>MKVTFEQLKAAFNRVLISRGVDSETADACAEMFARTTESGVYSHGVNRFPRFIQQLENGDIIPDAQPKRITSLGAIEQWDAQRSIGNLTAKKMMDRAIELAADHGIGLVALRNANHWMRGGSYGWQAAEKGYIGI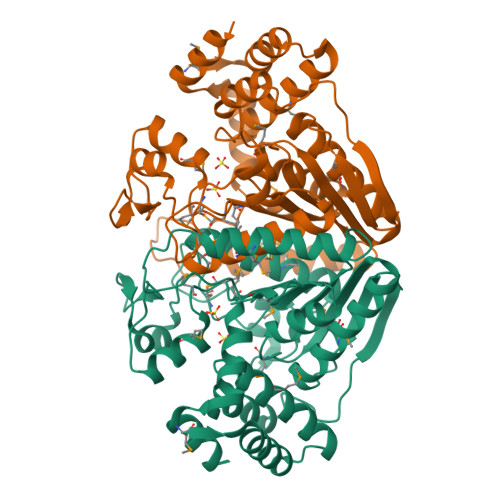CWTNSIAVMPPWGAKECRIGTNPLIVAIPSTPITMVDMSMSMFSYGMLEVNRLAGRQLPVDGGFDDEGNLTKEPGVIEKNRRILPMGYWKGSGMSIVLDMIATLLSDGASVAEVTQDNSDEYGISQIFIAIEVDKLIDGPTRDAKLQRIMDYVTSAERADENQAIRLPGHEFTTLLAENRRNGITVDDSVWAKIQALA[2x]> MAHHHHHHVDDDDKMVH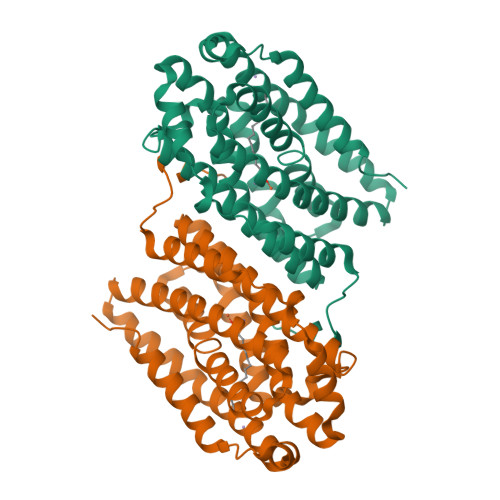HDGFQTVKATIDWEHPMFKLYEKAKRNGKWNPADIDFSQDQKDFASLTSEEKISALPLVAGFSAGEEAVTLDILPMAHALARQGRLEDVLFLTTFMHDEAKHVEMFSRWQQAVGIGQMDLSVFHNDHYKRIFYEALPEAMNRLYADDSPEAVIRAATVYNMIVEGTLAESGFYTFRQIYKKAGLFPGLLQGIDYLNMDEGRHIQFGIYTIQRIVNEDERYYELFIRYMDELWPHVIGYVDYLTELGKRQQQLARTYALEIDYDLLRHYVIKQFNLRKKQISRTKRVDVVEGLEKTAAES(4R)-5-IMINO-1-(5-O-PHOSPHONO-BETA-D-RIBOFURANOSYL)-4,5-DIHYDRO-1H-IMIDAZOLE-4-CARBOXYLIC ACID | C9 H14 N3 O9 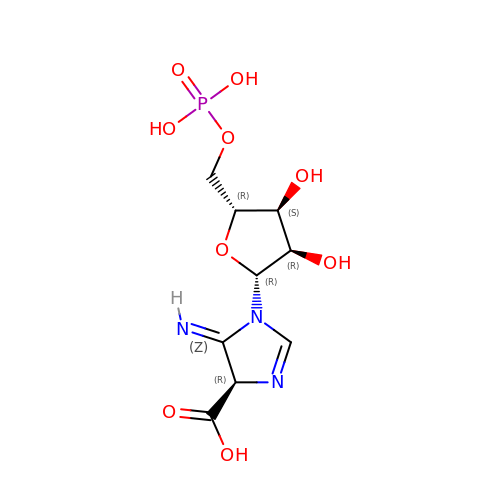P | WYRPDIVLQIXBHB-IUONDULESA-N>SLSLDEVIGEIIDLELDDQAISILEIKQEHVFSRNQIARGHHLFAQANSLAVAVIDDELALTASADIRFTRQVKQGERVVAKAK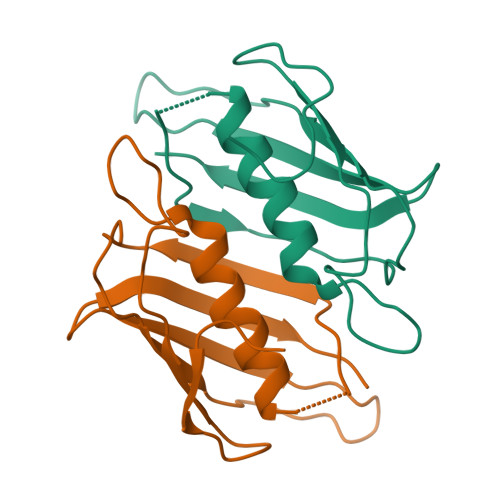VTAVEKEKGRTVVEVNSYVGEEIVFSGRFDMYRSKHS[4x]>MNLTELKNTPVSELIT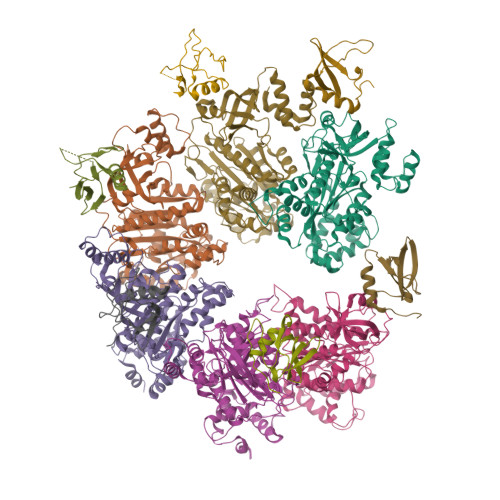LGENMGLENLARMRKQDIIFAILKQHAKSGEDIFGDGVLEILQDGFGFLRSADSSYLAGPDDIYVSPSQIRRFNLRTGDTISGKIRPPKEGERYFALLKVNEVNFDKPENARNKILFENLTPLHANSRLRMERGNGSTEDLTARVLDLASPIGRGQRGLIVAPPKAGKTMLLQNIAQSIAYNHPDCVLMVLLIDERPEEVTEMQRLVKGEVVASTFDEPASRHVQVAEMVIEKAKRLVEHKKDVIILLDSITRLARAYNTVVPASGKVLTGGVDANALHRPKRFFGAARNVEEGGSLTIIATALIDTGSKMDEVIYEEFKGTGNMELHLSRKIAEKRVFPAIDYNRSGTRKEELLTTQEELQKMWILRKIIHPMGEIDAMEFLINKLAMTKTNDDFFEMMKRS[6x];>[6x]MNDTYQPINCDDYDNLELACQHHLMLTLELKDGEKLQAKASDLVSRKNVEYLVVEAAGETRELRLDKITSFSHPEIGTVVVSES> MDIAKWVEHARTCYSTQLDTKIKVIGVIGKDYPDHGKGDNINCYLRENVFPVAATEDETCTIRGHFSEDDQILFLVMNGVDDVANIRKCLKSNPKSNYFDAMAESECQQIRMLHFLFISCHFIIIFEQTSRIDLELMRFLKKVNSARIQLRKKINQRLVASDLRDVSFNNRILSSAESEGRMVVPRLLIAFQRNNIRPDVNPGKKLQR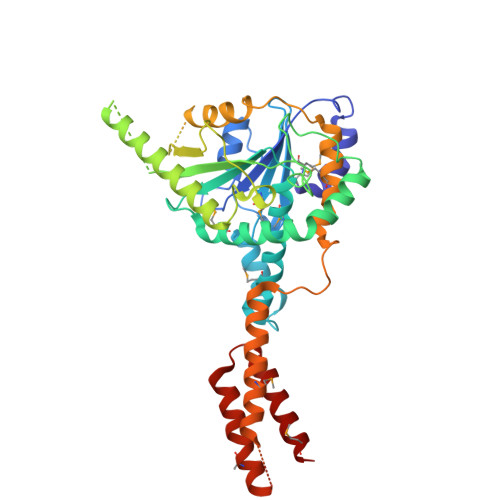ELYEKLEKNLDNQFSDILKLYDLIDCGASSLCQLNETIPVVHLLNPKIVKRDIIGEMFEILMADAENTKISGNAGTLPSNNSFVKFLEDNFRSEKNEISLENVIELMNCLQCVLDGDLEEKHEKTAIQTFIKRIQNDHMEEARRLYTNAQRPGERRGADRFKDSEKPVKIRSKEEHLMRFNEATHYIDSVVGVNSREALSQLQAQCNEMWQ> CELDRDPEGKDFQQPYTSFVQTKQNRDGLYALLRNTENPRMHFYQELQSDMYCTTITDGNSLAPFVNWDLGILNDHGRADEDEVSGIAGYYFVYNRLNQQANAFVNNTEAALQNQVYKNSTEIANAKSFLAEGKVLQALAIWRLMDRFSFHESVTEVNSGAKDLGVILLKEYNPGYIGPRATKAQCYDYILSRLSEAIEVLPENRESVLYVSRDYAYALRARIYLALGEYGKAAADAKMVVDKYPLIGAADAS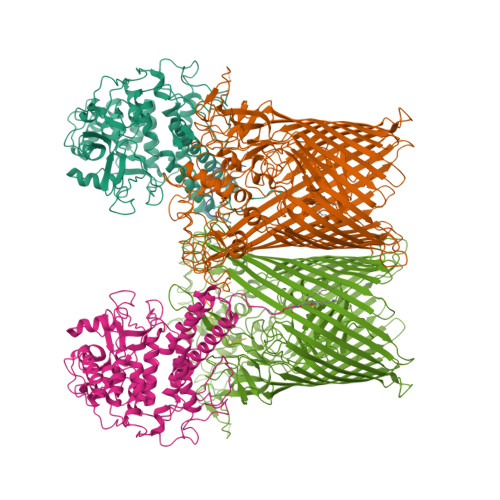EFENIYRSDANNPEIIFRGFASATLGSFTATTLNGAAPAGKDIKYNPSAVPFQWVVDLYENEDFRKSVYIAKVVKKDKGYLVNKFLEDKAYRDVQDKPNLKVGARYFSVAEVYLILVESALQTGDTPTAEKYLKALSKARGAEVSVVNMEALQAERTRELIGEGSRLRDMVRWSIPNNHDAFETQPGLEGFANTTPLKAQAPVGFYAYTWEFPQRDRQTNPQLIKNWPI;> QVVVLGYGTGQKLSTVSGSVAKVSSEKLAEKPVANIMDALQGQVAGMQVMTTSGDPTAVASVEIHGTGSLGASSAPLYIVDGMQTSLDVVATMNPNDFESMSVLKDASATSIYGARAANGVVFIQTKKGKMSERGRITFNASYGISQILNTKPLDNMMTGDELLDFQVKAGFWGNNQTVQKVKDMILAGAEDLYGNYDSLKDEYGKTLFPVDFNHDADWLKALFKTAPTSQGDISFSGGSQGTSYYASIGYFDQEGMAREPANFKRYSGRLNFESRINEWLKVGANLSGAIANRRSADYFGKYYMGSGTFGVLTMPRYYNPFDVNGDLADVYYMYGATRPSMTEPYFAKMRPFSSESHQANVNGFAQITPIKGLTLKAQAGVDITNTRTSSKRMPNNPYDSTPLGERRERAYRDVSKSFTNTAEYKFSIDEKHDLTALMGHEYIEYEGDVIGASSKGFESDKLMLLSQGKTGNSLSLPEHRVAEYAYLSFFSRFNYGFDKWMYIDFSVRNDQSSRFGSNNRSAWFYSVGGMFDIYNKFIQESNWLSDLRLKMSYGTTGNSEIGNYNHQALVTVNNYTEDAMGLSISTAGNPDLSWEKQSQFNFGLAAGAFNNRLSAEVDFYVRTTNDMLIDVPMPYISGFFSQYQNVGSMKNTGVDLSLKGTIYQNKDWNVYASANFNYNRQEITKLFFGLNKYMLPNTGTIWEIGYPNSFYMAEYAGIDKKTGKQLWYVPGQVDADGNKVTTSQYSADLETRIDKSVTPPITGGFSLGASWKGLSLDADFAYIVGKWMINNDRYFTENGGGLMQLNKDKMLLNAWTEDNKETDVPKLGQSPQFDTHLLENASFLRLKNLKLTYVLPNSLFAGQNVIGGARVYLMARNLLTVTKYKGFDPEAGGNVGKNQYPNSKQYVAGIQLSF;> GTGGSTGTTSAG> PVNTKRSNGTKRVEFPTTKKSMCIGNSTPNEQETFRAKVDEIWFRLTQKTDGTVMRDFLIEKAAEYFKQPEQPKQNAIEVISAIMAPQEEQTKSKADLYKFLAMFGPYETIMLKIASL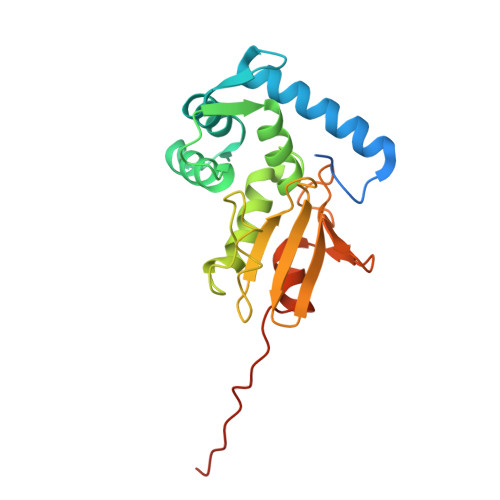LLISNNKGHWLTFDPQAEKNANNQRDSISGWFDQNEPNCLILKTPTGIRKIWNKPLIEATGQYLMDENGEKYDSWDKYFEMKPIETYLTAYPTFAPMHHHHHH> MGTQLVMYEEEFTKINAVCDRLTKDANAKVVFLVDKNGQLISSAGQTQNIDTTS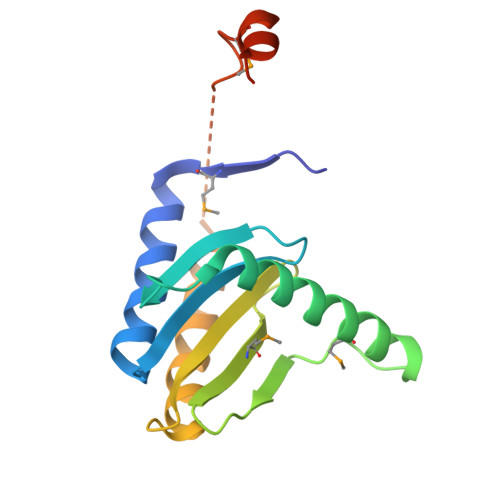LASLTAGNVAAMGGLAKLIGENEFPNQFHEGAKDSLYMTIVGSRVVLVVIFDNRTSLGLVRLRIKKASDELTKIFESLVKKTDSPGAGSPFAEMSDDDIDNLFSEGSHHHHHH> DQTQKAAAE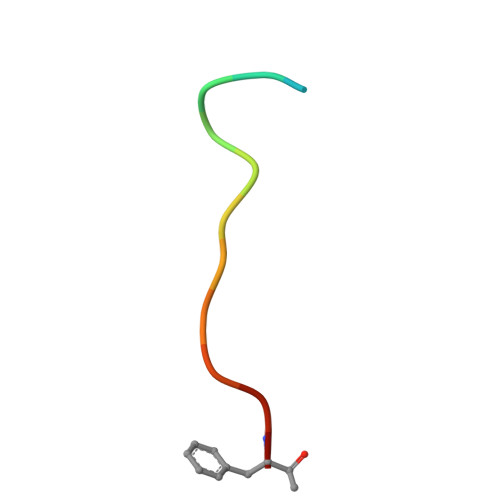LTFFX>[2x]MERAIQGNDTREQANGERWDGGSGGITSPFKLPDESPSWTEWRLYNDETNSNQDNPLGFKESWGFGKVVFKRYLRYDRT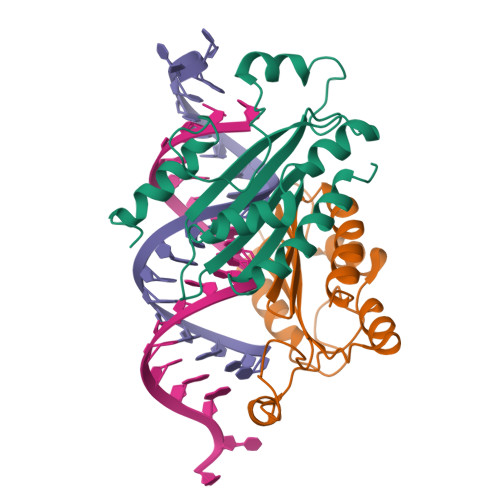EASLHRVLGSWTGDSVNYAASRFLGANQVGCTYSIRFRGVSVTISGGSRTLQHLCEMAIRSKQELLQLTPVEVESNVSRGCPEGIETFKKESE>[2x]GHMNDALHIGLPPFLVQANNEPRVLAAPEARMGYVLELVRANIAADGGPFAAAVFERDSGLLIA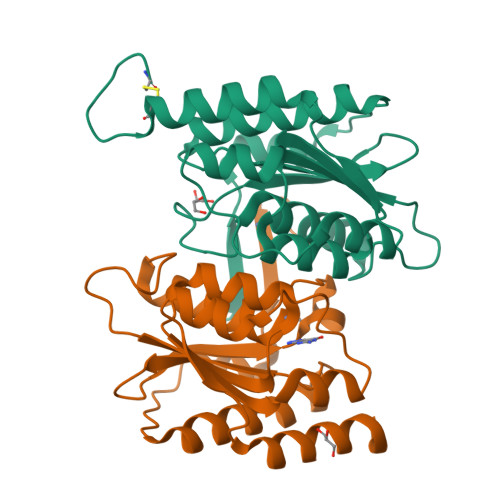AGTNRVVPGRCSAAHAEILALSLAQAKLDTHDLSADGLPACELVTSAEPCVMCFGAVIWSGVRSLVCAARSDDVEAIGFDDGPRPENWMGGLEARGITVTTGLLRDAACALLREYNACNGVIYNARCGVHK> QTARKST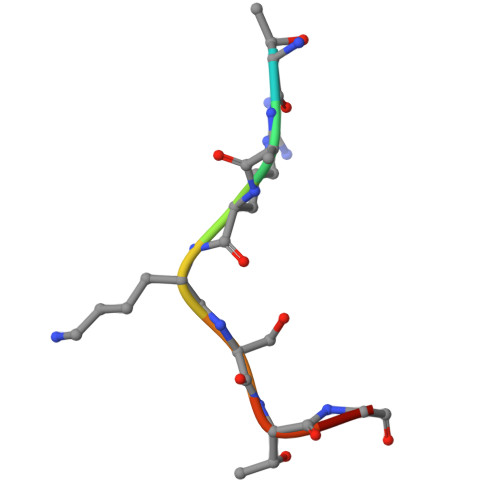GG> SNAMALKKPGSLTIAGSGIASIGHITLETLALIKEADKIFYAVTDPATECYIQENSRGDHFDLTTFYDTNKKRYESYVQMSEVMLRDVRAGRN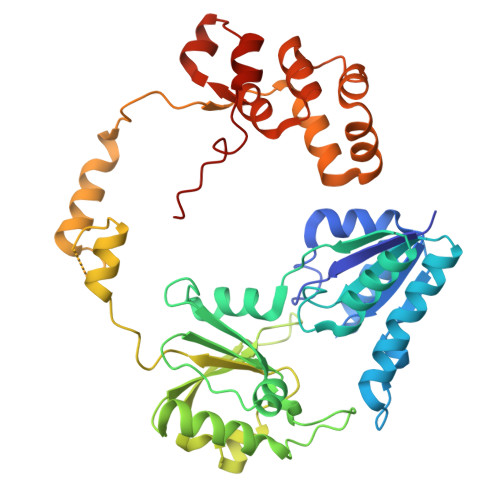VLGIFYGHPGVFVAPSHRAIAIAREEGFQAKMLPGISAEDYMFADLGFDPSTYGCMTQEATELLVRNKKLDPSIHNIIWQVGSVGVDTMVFDNGKFHLLVERLEKDFGLDHKIQHYIGAILPQSVTVKDTFAIRDLRKEEVLKQFTTTSTFYVPPRTPAPIDPKAVQALGLPATVTKGAQDWTGFQSVSPAYGPDEMRAVAALDSFVPSQEKAVVHASRAMQSLMVDLALRPALLEQYKADPVAFANTRNGLTAQEKFALGLKKPGPIFVVMRQLPSAIASGQEPSQEEIARADDATAFIIIYIVQG[4-(5-naphthalen-2-yl-1H-pyrrolo[2,3-b]pyridin-3-yl)phenyl]acetic 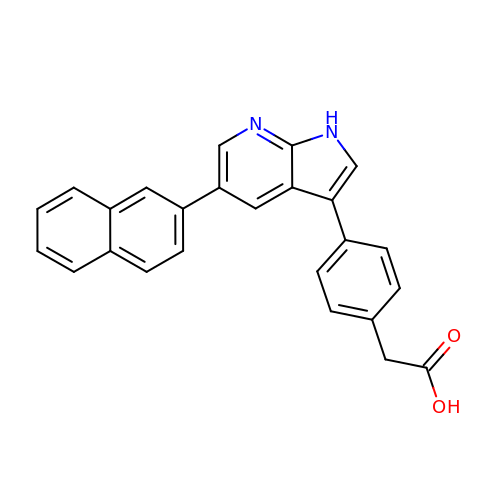acid | C25 H18 N2 O2 | SWXKLXXVFMYMDP-UHFFFAOYSA-N> MVPISPIETVPVKLKPGMDGPKVKQWPLTEEKIKALVEICTELEKEGKISKIGPENPYNTPVFAIKKKNSTRWRKLVDFRELNKRTQDFWEVQLGIPHPAGLKKKKSVTVLDVGDAYFSVPLDEDFRKYTAFTIPSINNETPGIRYQYNVLPQGWKGSPAIFQSSMTKILEPFKKQNPDIVIYQYMDDLYVGSDLEIGQHRTKIEELRQHLLRWGLYTPDQKHQKEPPFLWMGYELHPDKWTVQPIVLPEKDSWTVNDICKLVGKLNWASQIYPGIKVRQLSKLLRGTKALTEVIPLTEEAELELAENREILKEPVHGVYYDPSKDLIAEIQKQGQGQWTYQIYQEPFKNLKTGKYARMRGAHTNDVKQLTEAVQKITTESIVIWGKTPKFKLPIQKETWETWWTEYWQATWIPEWEFVNTPPLVKLWYQLEKEPIVGAETFYVDGAANRETKLGKAGYVTNKGRQKVVPLTNTTNQKTELQAIYLALQDSGLEVNIVTDSQYALGIIQAQPDKSESELVNQIIEQLIKKE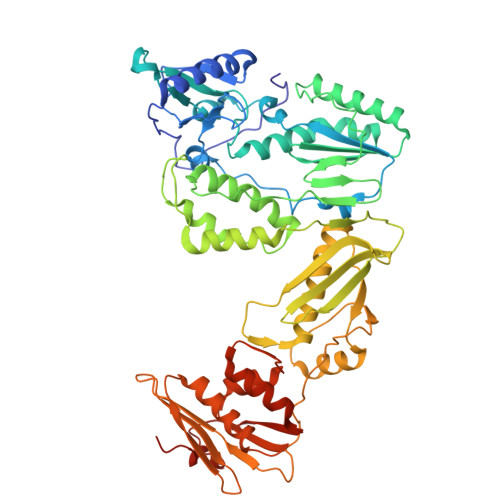KVYLAWVPAHKGIGGNEQVDKLVSAGIRKVL>DDEIDREHQERNAEISACNARALSEGRPASLVYLSR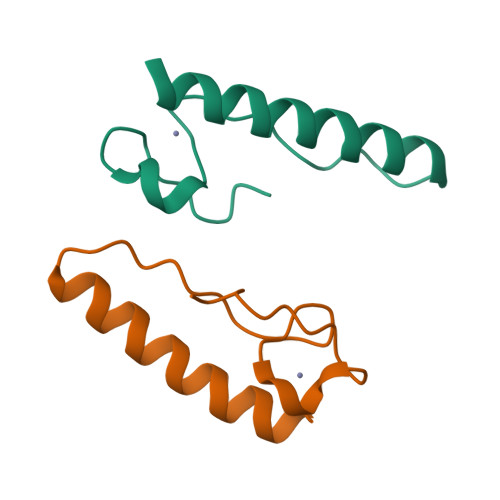DACDIPEHSGRCRFVKYLNF[2x]> GSHMGEGEGVQLTAAQELMIQQLVAAQLQSNKRSFSDQPKVTPWPLGADPQSRDARQQRFAHFTELAIISVQEIVDFAKQVPGFLQLGREDQIALLKASTIEIMLLET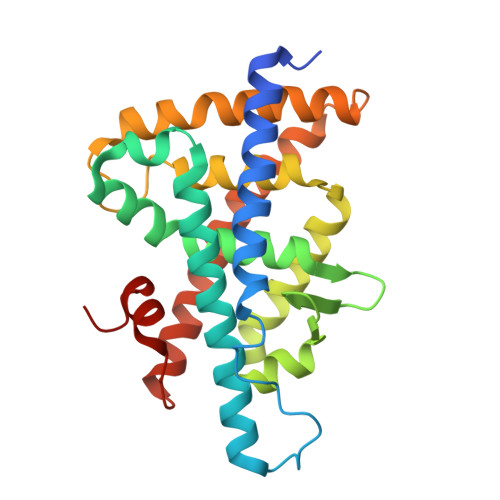ARRYNHETESITFLKDFTYSKDDFHRAGLQVEFINPIFEFSRAMSSLGLDDAEYALLIAINIFSADRPNVQEPGRVEALQQPYVEALLSYTRIKRPQDQLRFPRMLMKLVSLRTLSSVHSEQVFALRLADAALPPLLSEIWDVHE>MDLHSLLELGTKPTAPHVRNKKVILFDTNHQVSICNQIIDAINSGIDLGDLLEGGLLTLCVEHYYNSDKDKFNTSPIAKYLRDAGYEFDVIKNADATRFLDVIPNEPHYSPLILALKTLESTESQRGRIGLFLSFCSLFLPKLVVGDRASIEKALRQVTVHQEQGIVTYPNHWLTTGHMKVIFGILRSSFILKFVLIYQGVNLVTGHDAYDSIISNSVGQTRFSGLLIVKTVLEFILQKTDSGVTLHPLVRTSKVKNEVASFKQALSNLARHGEYAPFARVLNLSGINNLEHGLYPQLSAIALGVATAH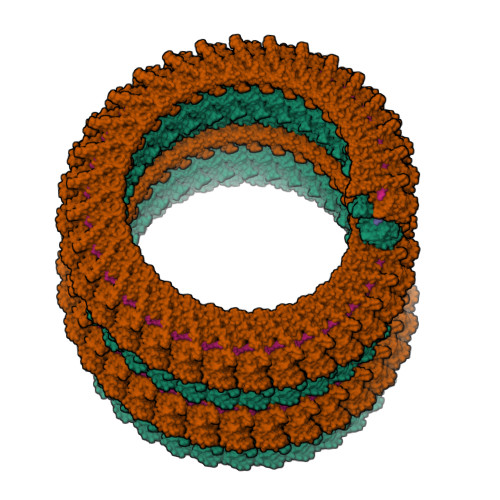GSTLAGVNVGEQYQQLREAAYDAEVKLQRRHEHQEIQAIAEDDEERKILEQFHLQKTEITHSQTLAVLSQKREKLARLAAEIENNI[2x]>[6x]GGGGRSVDTMALWLGLRAVLVVAGLAVLLQLIRGWLSSKSYVFNREEIARLAKEHSGLDYEVAFSKIIVELRKKHPGHILQDEDLQWVFVNAGGWMGSMCLLHASLTEYVLLFGTAVDTGGHSGRYWAEISDTILSGTFRQWKEGTTKSEIFYPGDTIVHEVGEATSVQWSSGTWMVEYGRGFIPSTLAFALADTIFSTQDFLTLFYTVKVYSKALLLEASTHLSQLGFFAAA

The sigma-1 receptor (σ1R) is an endoplasmic reticulum (ER)-localized, non-opioid transmembrane receptor implicated in many pathological conditions, including neurodegenerative disorders and cancer. So far, all reported σ1R structures are homotrimers, with the ligand binding site located inside the β-barrel domain of each σ1R monomer. The ligand binding site is located in the lumen of the β-barrel domain (β1-β10), whose opening is covered by two membrane-adjacent helices (α4/α5) at the carboxy-terminus. Here, we present crystal structures of σ1R from Xenopus laevis (xlσ1R) bound to two endogenous neurosteroid ligands, progesterone (a putative antagonist) and dehydroepiandrosterone sulfate (DHEAS) (a putative agonist), at 2.15-3.09  Å resolutions.

Recently, we determined another xlσ1R-DHEAS complex structure to 3.09  Å in a C2 form (termed xlσ1RDHEAS-C2). The xlσ1RDHEAS-C2 structure contains six protomers (two trimers) in an asymmetric unit. These protomers aligned well between each other and with xlσ1RDHEAS-I432. Interestingly, DHEAS seems to show three different binding poses in xlσ1RDHEAS-C2: Pose-1 for protomers A and D, Pose-2 for protomers B, E and F (also for xlσ1RDHEAS-I432), and Pose-3 for protomer C. The three DHEAS poses differ mainly in that the C3 sulfuric ester group assumes different conformations. This data may provide potential evidence of flexible (and possibly loose) binding of DHEAS’ C3 sulfuric ester group in the distal β-barrel lumen region of xlσ1R. Meanwhile, due to the resolution limit of xlσ1RDHEAS-C2 (3.09  Å), which may not be sufficient to distinguish clearly different conformations of the sulfate group of DHEAS, we interpreted the xlσ1RDHEAS-C2 structure with caution and used it only as supplemental evidence to discuss DHEAS binding in xlσ1R.> TVSVLLPFVATEFYRRLVEGIEGVLLEQRYDLALFPILSLARLKRYLENTTLAYLTDGLILASYDLTERFEEGRLPTERPVVLVDAQNPRYDSVYLDNRLGGRLAGAYLARFPGPIFAIAVEEEPDRAFRRTVFAERMAGFQEALKEAGRPFSPDRLYITRHSQEGGRLALRH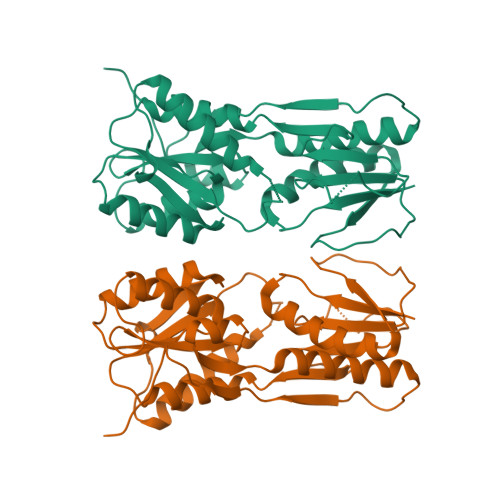FLEKASPPLNVFAGADQVALGVLEEAVRLGLTPGRDVRVLGFDGHPFAEEAGLSTIAQPVEAMGARAAQLLLERMRGYQGPPREVRFEPVLVERASTGTPPAA In addition to housekeeping NusG, diverse bacterial paralogs, typified by E. coli RfaH, activate long operons that encode antibiotics, capsules, toxins, and pili by inhibiting Rho-dependent termination, an activity inverse to that of NusG. RfaH-CTD, unlike the CTDs of all other known NusG/Spt5 proteins, which adopt a β-barrel structure, folds as an α-helical hairpin that masks the RNAP-binding site on the NTD. RfaH is recruited at ops sites in vitro and in vivo through direct contacts with the non-template (NT) DNA strand in the transcription bubble, a target shared with σ. Contacts with the ops element in the NT DNA are thought to trigger domain dissociation, transforming RfaH into an open, active state in which the NTD can bind to RNAP; consistently, destabilization of the domain interface enables sequence-independent recruitment.

To visualize the molecular details of RfaH:DNA interactions, we determined a crystal structure of RfaH bound to a 9-nt ops DNA encompassing bases G2 – G10 (ops9) at a resolution of 2.1 Å. The DNA binds to a basic patch on RfaH-NTD opposite the RNAP/RfaH-CTD binding site and forms a hairpin structure. The hairpin loop comprises G4-A7, with T6 flipped out so that its nucleobase is completely exposed. Flipped T6 inserts into a deep, narrow, positively charged pocket on RfaH-NTD, which is mainly formed by H20, R23, Q24, and R73 located in helices α1 and α2. RfaH-NTD exclusively contacts nucleotides in the loop region, involving K10, H20, R23, Q24, T68, N70, A71, T72, R73, G74, and V75. Base-specific interactions with RfaH-NTD are made by G4, G5, and T6; however, only G5 and T6 form a hydrogen-bond network with RfaH-NTD that may underlie sequence-specific recognition. Thus, contacts between only two nucleobases and four amino acids mediate specific recognition of ops by RfaH. The stem of the DNA hairpin is formed by base pairs C3:G8 and G2:C10, with T9 being flipped out. The G2:C10 base pair is likely an artifact of crystal packing as the stems of neighboring DNA molecules stack on each other and could not form in a TEC that contains a 10–11 nt bubble. However, this idea is refuted by our observations that domain interface remains intact in the binary complex, implying that additional interactions with RNAP or nucleic acids relieve autoinhibition.

>MQSWYLLYCKRGQLQRAQEHLERQAVNCLAPMITLEKIVRGKRTAVSEPLFPNYLFVEFDPEVIHTTTINATRGVSHFVRFGASPAIVPSAVIHQLSVYKPKDIVDPATPYPGDKVIITEGAFEGFQAIFTEPDGEARSMLLLNLINKEIKHSVKNTEFRKA[2x]>[12x]MSSNAIGLIETKGYVAALAAADAMVKAANVTI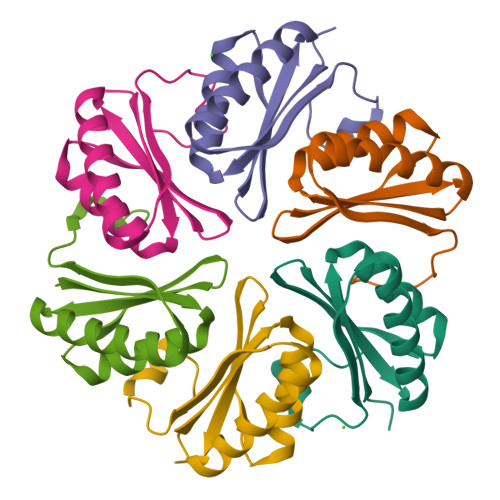TDRQQVGDGLVAVIVTGEVGAVKAATEAGAETASQVGELVSVHVIPRPHSELGAHFSVSSKLEHHHHHH Tailed bacteriophages and herpesviruses use a transient scaffold to assemble icosahedral capsids with hexameric capsomers on the faces and pentameric capsomers at all but one vertex where a 12-fold portal is thought to nucleate the assembly. We have determined the portal vertex structure of the bacteriophage HK97 procapsid, where the scaffold is a domain of the major capsid protein. Assembly of this large complex from hundreds of protein subunits requires transient association of an internal scaffolding protein or domain that acts similar to a chaperone and is absent from the mature capsid. The mcp gene 5 encodes a 103-residue N-terminal scaffolding domain (mcpN) and a 281-residue C-terminal domain (mcpC) that exhibits the HK97-fold including a triangular A-domain; a P-domain, composed of a long spine α helix; an adjacent three-stranded β sheet; the flexible E-loop; and the N-arm.

The asymmetric reconstruction of the portal vertex shows that the portal and surrounding capsomer density were equally well defined, indicating that the portal and the five surrounding hexons have a unique mutual orientation. The portal clip domains visible from the exterior exhibit neither strict 12-fold nor 5-fold symmetry, suggesting that the 12 portal subunits adjust to their incongruent fivefold environment. Besides the clip domain, the portal density exhibits strict 12-fold symmetry and the 10 towers of mcpN interact at symmetrically equivalent positions on the side of the portal (right), but leaving two specific positions unoccupied. Visualized from the capsid interior, these stripes correspond to ten ~100-Å-long towers that surround the portal and originate from the surrounding capsomers, two towers per hexon. The towers were readily modeled as trimeric coiled coils consistent with residues 2 to 66 from mcpN and accounted for all 30 scaffold domains around the portal. Thus, the scaffolding domains adopt a pseudo-12-fold organization, buffering the 12 to 5 symmetry mismatch at this special vertex. Cross sections along the portal axis showed that the portal/mcp interaction is mediated by mcpN, including some of the surrounding S76 to S88 α helix but primarily by the flexible spacers and coiled coils that adhere to the portal’s 12-fold symmetry. Our model of the portal, despite lacking 50 N-terminal residues that are not visible in the density map, revealed several contacts with the scaffold that occur in a groove between the wing domains of two portal subunits in Fig. 6B. We observed that only one of the three coiled-coil helices interacts in this groove where it is surrounded by a polar distribution of charges: lysines (156, 160, 161, and 346) from one portal subunit and aspartates (94, 135, 141, and 169) from the other. We show that no less than 30 mcpN domains interact directly with the portal.

>MEEPKYTIDLRTNNGWWARLKSWFVGGRLVTPNQGSQTGPVSAHGYLGDSSINDERILQISTVWRCVSLISTLTACLPLDVFETDQNDNRKKVDLSNPLARLLRYSPNQYMTAQEFREAMTMQLCFYGNAYALVDRNSAGDVISLLPLQSANMDVKLVGKKVVYRYQRDSEYADFSQKEIFHLKGFGFTGLVGLSPIAFACKSAGVAVAMEDQQRDFFANGAKSPQILSTGEKVLTEQQRSQVEENFKEIAGGPVKKRLWILEAGFSTSAIGVTPQDAEMMASRKFQVSELARFFGVPPHLVGDVEKSTSWGSGIEQQNLGFLQYTLQPYISRWENSIQRWLIPSKDVGRLHAEHNLDGLLRGDSASRAAFMKAMGESGLRTINEMRRTDNMPPLPGGDVAMRQAQYVPITDLGTNKEPRNNGA[12x]>PTSPFETLRAAAAPRYFGAALGVPHLLNFTHDPLFDVTAVLQFNGATPENEMKWAYIEPERNQFNFTGGDIVAAFSAANDYVLRGHNLVWYQELAPWVETLT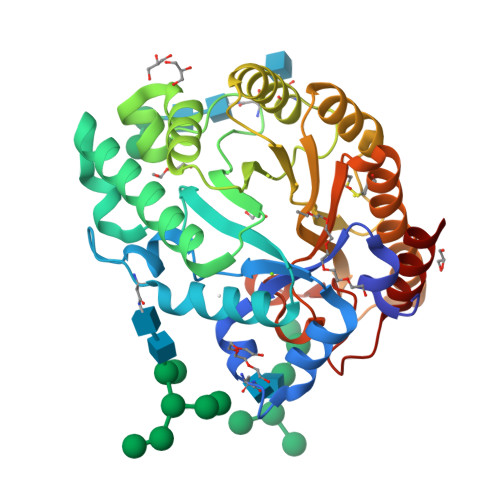GEDLWNATVNHITTVMTHYKESFNIYAWDVVNEAFNDNGTYRENVWYTQLGPDYIPNAYAVARSVNTPSKLYINDYNTEGINNKSDALLAVVQSMKAHNLVDGVGFQCHFFVGELPPDLEQNFARFVAAGVEIAVTELDIRMNLPPSQADIEQQARDYATVVNACKAQGAACVGITTWGITDLYSWIPSTYPGEGYALLFDDNYVPHPAFNATIQALLA[2x]> SRMQLSEEQAAVLRAVLKGQSIFFTGSAGTGKSYLLKRILGSLPPTGTVATASTGVAACHIGGTTLHAFAGIGSGQAPLAQCVALAQRPGVRQGWLNCQRLVIDEISMVEADLFDKLEAVARAVRQQNKPFGGIQLIICGDFLQLPPVTKGSQPPRFCFQSKSWKRCVPVTLELTKVWRQADQTFISLLQAVRLGRCSDEVTRQLQATASHKVGRDGIVATRLCTHQDD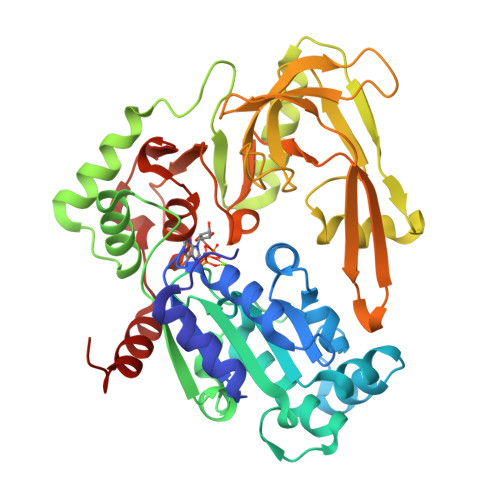VALTNERRLQELPGKVHRFEAMDSNPELASTLDAQCPVSQLLQLKLGAQVMLVKNLSVSRGLVNGARGVVVGFEAEGRGLPQVRFLCGVTEVIHADRWTVQATGGQLLSRQQLPLQLAWAMSIHKSQGMTLDCVEISLGRVFASGQAYVALSRARSLQGLRVLDFDPMAVRCDPRVLHFYATLRRGRSL> YFQ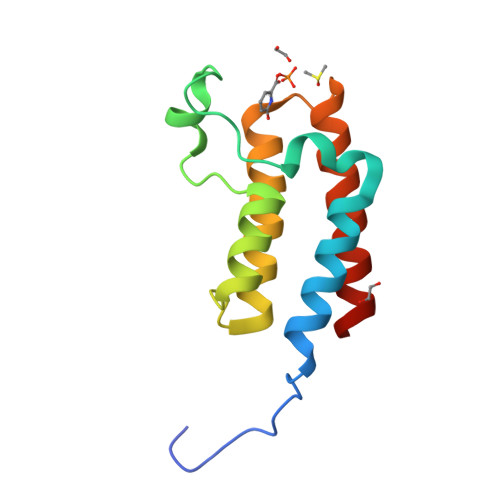SMSVKKPKRDDSKDLALCSMILTEMETHEDAWPFLLPVNLKLVPGYKKVIKKPMDFSTIREKLSSGQYPNLETFALDVRLVFDNCETFNEDDSDIGRAGHNMRKYFEKKWTDTFKVS> GSHMGSNQKRGVKVLKQELGGLGISIKGGKENKMPILISKIFKGLAADQTQALYVGDAILSVNGADLRDATHDEAVQALKRAGKEVLLEVKYMREGSAYGSVKAYTNFDAERDALNIETAIKTKGVDEVTIVNILT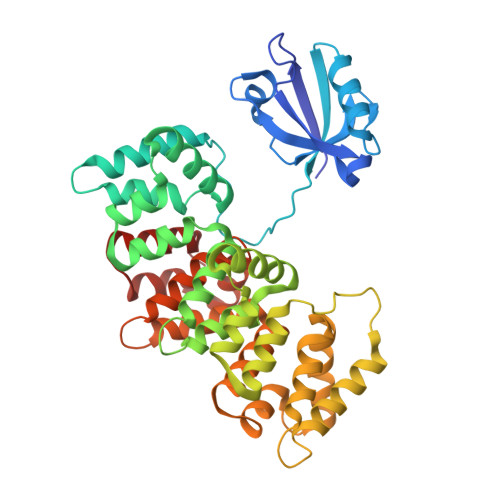NRSNEQRQDIAFAYQRRTKKELASALKSALSGHLETVILGLLKTPAQYDASELKASMKGLGTDEDSLIEIICSRTNQELQEINRVYKEMYKTDLEKDIISDTSGDFRKLMVALAKGRRAEDGSVIDYELIDQDARDLYDAGVKRKGTDVPKWISIMTERSVPHLQKVFDRYKSYSPYDMLESIRKEVKGDLENAFLNLVQCIQNKPLYFADRLYDSMKGKGTRDKVLIRIMVSRSEVDMLKIRSEFKRKYGKSLYYYIQQDTKGDYQKALLYLCGGDD> MRGSHHHHHHGSMAVPPTYADLGESARDVFTKGYGFGLIKLDLKTKSENGLEFTSSGSANTETTKVNGSLETKYRWTEYGLTFTEKWNTDNTLGTEITVEDQLARGLKLTFDSSFSPNTGKKNAKIKTGYKREHIN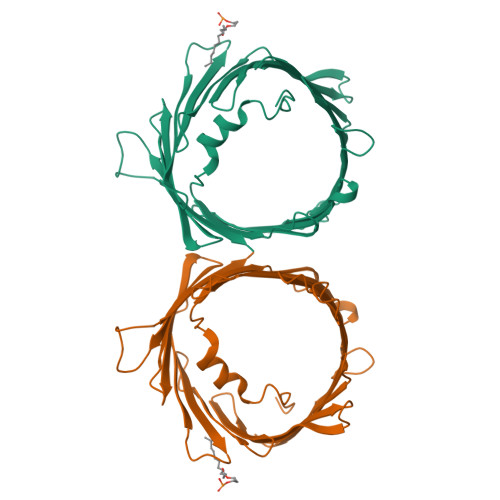LGCDVDFDIAGPSIRGALVLGYEGWLAGYQMNFETSKSRVTQSNFAVGYKTDEFQLHTNVNDGTEFGGSIYQKVNKKLETAVNLAWTAGNSNTRFGIAAKYQVDPDACFSAKVNNSSLIGLGYTQTLKPGIKLTLSALLDGKNVNAGGHKLGLGLEFQA> MKKYHISMINIPAYGHVNPTLALVEKLCEKGHRVTYATTEEFAPAVQQAGGEALIYHTSLNIDPKQIREMMEKNDAPLSLLKESLSILPQLEELYKDDQPDLIIYDFVALAGKLFAEKLNVPVIKLCSSYAQNESFQLGNEDMLKKIREAEAEFKAYLEQEKLPAVSFEQLAVPEALNIVFMPKSFQIQHETFDDRFCFVGPSLGERKEKESLLIDKDDRPLMLISLGTAFNAWPEFYKMCIKAFRDSSWQVIMSVGKTIDPESLEDIPANFTIRQSVPQLEVLEKADLFISHGGMNSTMEAMNAGVPLVVIPQMYEQELTANRVDELGLGVYLPKEEVTVSSLQEAVQAVSSDQELLSRVKNMQKDVKEAGGAERAAAEIEAFMKKSAVP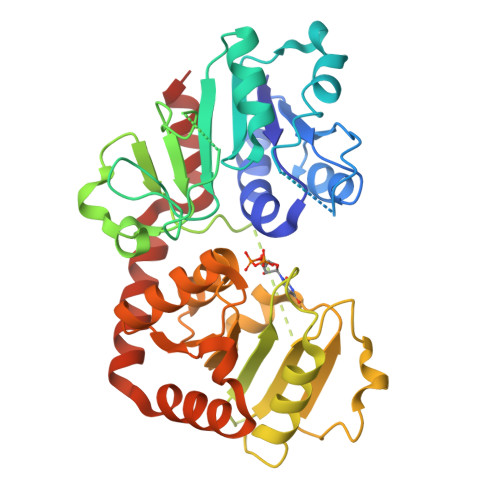Q>MSAHRTLLLRLSDSGEPVTSCSYGQGVLTLPSLPLPQGKKLGDMPVYTVKLAIPAGSPVTRDGLIWTNCPPDFSTQFDREKFYKKIIKTSFHEDDHIDLDIYVPGTYCFYLSFKNDKDELETTRKFYFVVLPILSVNDKFIPLNSIAMQSVVSKWMGPTIKDWEKVFARVASKKYNMIHFTPLQHRGESNSPYSIYDQLEFDPTVFKSEKEVADMVERLRTEHNILSLTDIVFNHTANNSQWLLDHPEAGYNHKTSPHLISAIELDKKLLDFSEQMEALGYPVDLKTVDDLIKVMDGIKEHVIGELKLWEFYVVDVKQTVSELREKWGNSKSWSDDNIPSKDDSTNLAQFVRDNATEPGFGSLGERGSNKINIDKFAAILKKLHSEDYNNGIEELATKILNDINLPFYKEYDDDINEVLEQLFNRIKYLRIDDHGPKQGPITKKLPLSEPYFTRFKAKDGEEYALANNGAIWDGNPLVDFASSQSKAYLRREVIVWGDCVKLRYGKGPSDSPYLWERMSKYVEMNARIFNGFRIDNCHSTPLHVGQYFLDVARRVNPNLYVVAQLFSGSEAMDCLFVERLGISSLIREAMQAWSEEELSRLVHRHGGRPIGSYKFVPLDDFPYPADVKIDEEYCAYNPDDHSVKCVSEIMIPKTLTATPPHALFMDCTHDNETPNQKRTVEDTLPNAALVAFCSSAIGSVYGYDEVFPQLLDLVQEKRTYSCAENTGISKVKTLLNNMREEIASEAVDIEDSEMHVHHDGQYITFHRTNAKNGKGWYLVARTKFHSSGDQMLPRIKLSQTKATFKAAFSLERTGDAPISDEIIEGIPTKLRELTGFDIGFDENTKETSILLPQDFPQGSIVIFETQQLGIDDSLDHFIRSGAIKATEKLSLESINYVLYRAEQEEYDYSEGRSGAYDIPDYGKPVYCGLQGWVSILRKIIFYNDLAHPLSNNLRNGHWAVDYVVNRLDLYKDKEGVAEVQEWLRSRMERIKQLPSYLVPSFFALVVGIMYGCCRLRAMQLMSDNVGKSTVFVQSLAMTSIQMVSAMKSTSILPDQNIAAMAAGLPHFSTNYMRCWGRDVFISLRGLLLTTGRYEEAKEHILAFAKTLKHGLIPNLLDAGRNPRYNARDAAWFFVQAIQDYVTIVPGGVSLLQEKVTRRFPLDDEYIPYDDPKAFSYSSTIEEIIYEILNRHAGGIKYREANAGPNLDRVMKDEGFNVEVNVDWETGLIHGGSQFNCGTWMDKMGESEKANSVGVPGTPRDGAAVEINGLLKSCLRFVLQLSKDGKFKYTEVTKPDGSKISLSSWNDLLQENFERCFYVPKNKEDDNKFEIDATIINRRGIYKDLYRSGKPYEDYQFRPNFTIAMVVAPELFTPDYAAGAIELADQVLRGPVGMRTLDPSDYNYRPYYNNGEDSDDFATSKGRNYHQGPEWVWCYGYFIRAYHYFNFLTNPKCQVEGSAKKLKPSSYLYRKLYSRLLKHREWIENSPWAGLAELTNKDGEVC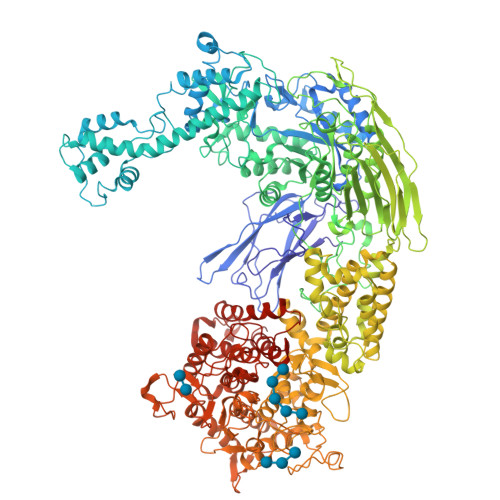NDSSPTQAWSTGCLLDLFYDLWISYEELEHHHHHH[2x]1-(4-chlorophenyl)-6,6-dimethyl-1,6-dihydro-1,3,5-triazine-2,4-diamine | C11 H14 Cl N5 | 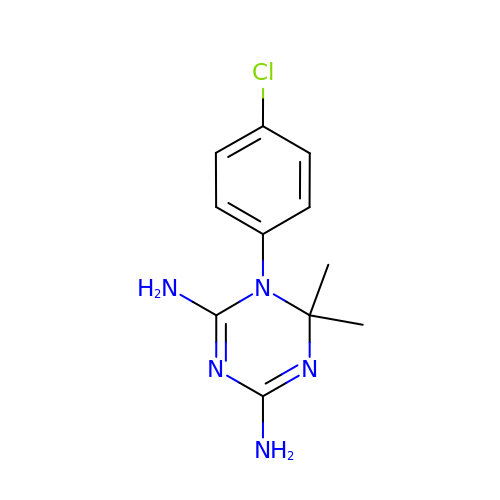QMNFFXRFOJIOKZ-UHFFFAOYSA-N>ELPQMTQQLNSDDMQEQLSATVKFRQILSREHRPPIDVVIQAGVVPRLVEFMRENQPEMLQLEAAWALTNIASGTSAQTKVVVDADAVPLFIQLLYTGSVEVKEQAIWALGNVAGDSTDYRDYVLQCNAMEPILGLFNSNKPSLIRTATWTLSNLCRGKKPQPDWSVVSQALPTLAKLIYSMDTETLVDACWAISYLSDGPQEAIQAVIDVRIPKRLVELLSHESTLVQTPALRAVGNIVTGNDLQTQVVINAGVLPALRLLLSSPKENIKKEACWTISNITAGNTEQIQAVIDANLIPPLVKLLEVAEDKTKKEACWAISNASSGGLQRPDIIRYLVSQGCIKPLCDLLEIADNRIIEVTLDALENILKMGEADKEARGLNINENADFIEKAGGMEKIFNCQQNENDK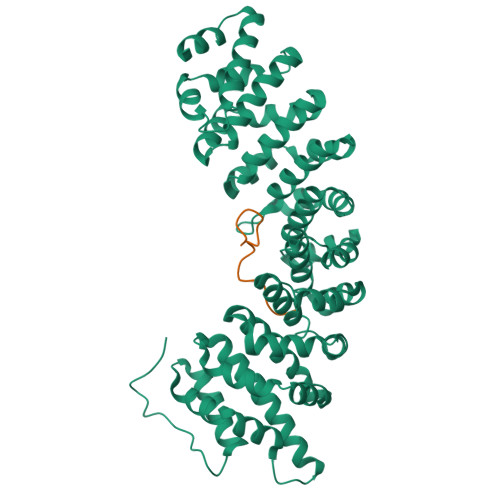IYEKAYKIIETYFGEEEDAVDETMAPQNAGNTFG[2x];>MAKRVADAQIQRETYDSNESDDDVTPSTKVASSAVMNRRKIAMPKRRMAFK[2x]>IEKQMDRVVKEMRRQLEMIDKLTTREIEQVELLKRIYDKLTVQ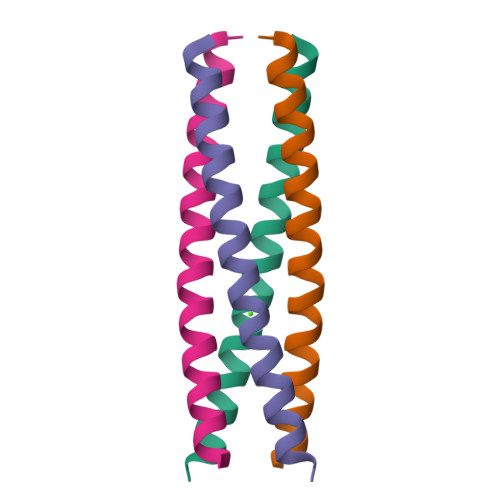TTGEIDMTK[2x]> GSPNSPATGEKKECWSWESYLEEQKAITAPVSLFQDSQAVTHNKNGFKLGMKLEGIDPQHPSMYFILTVAEVCGYRLRLHFDGYSECHDFWVNANSPDIHPAGWFEKTGHKLQPPKGYKEEEFSWSQYLRSTRAQAAPKHLFVSQSHSPPPLGFQVGMKLEAVDRMNPSLVCVASVTDVVDSRFLVHFDNWDDTYDYWCDPSSPYIHPVGWCQKQGKPLTPPQDYPDPDNFCWEKYLEETGASAVPTWAFKVRPPHSFLVNMKLEAVDRRNPALIRVA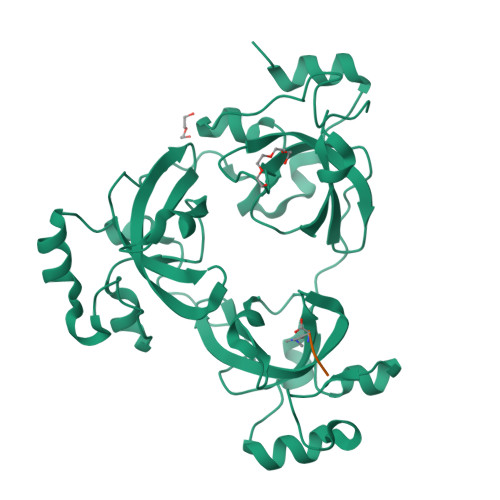SVEDVEDHRIKIHFDGWSHGYDFWIDADHPDIHPAGWCSKTGHPLQPPLGPREPSSAVDSSGRIVTD;> KATKK>TLLCGEIHYFRVPKHLWRDRLLKLKRAGGNCVSTYIPWNWHDPREKVVNFTDGTSQWHVASYYSRDLASFLELAGELGLRVIARPGPYICSEWDSGGHPNWIYTKAMRLRSLDPGYFKHVVEWYNSVLNILKPYVEREIVIGIQVENEYFWGNEKYIEKLAEIVEEKLPGVLVFTNEDPYLTRIPNTIDLYPSPWDMRQFDDRLRSYLSSQPGLFKMIMELEGGWFKSSRYGYYPTNRLSIPPEWTEILLKTAVGMGLNNINIYMFHGGSNPGYYTAKYLASSYDFEACIREWGELSERYYRVKRVFTFLNGFQELVTSLKPGETVKTASTCSELLQRVGDHGKIAVLRNTGDNLCYQRLINRGEIIPMWTPIRVPPRYAKIVLLDLVVEGTPFKLVYTSGEALLMKRLGDTVVMIIYGDHGEYTETAVEVEGGVLDVDIQGDVLIRREGERAYLVVNHTHGEHLAIVKSTRGQNLLLIFTCRCRAEKTWIVDEDLVLISNIYYIGDSRIDEGKVVINAELDEDSCGRLLVVTSREIEAISLEDLDLDLTRLSKYVYATHIPLSMCRSGKNTYHPLEYRLLEDPVFHTLTSINPSSPLLKNGFYENGIYVYRLRLHLDKKQLGDLLDKHLALIG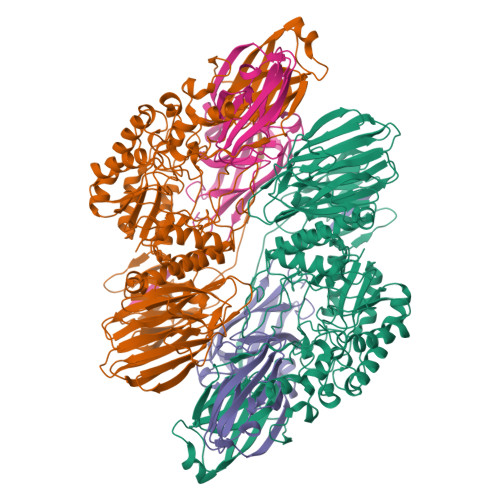FSDYAVVSINNEYAGSGYHYIEMSADSLREGVNEVTVILESTGHPNDGLLYVPNGIYGGVYLGRVGEIRLYKWRKTGFEIPYGPGFDLAEFIANPEPVIKALQE[2x];>ETYSVDSPGLYITEFKVDDLSRHYVLDPGLEFYYNHYYRILLFVNKVYVGPLIGPIDITRYLKPGVNEVALLVEWGVVNPVIGVYQYKVDGEWFIQEGLHGLIEEWFRRSPRGETAEPPILLGDKAGRVIWVNTVIPYEKEPTSSSPVKLEVDFWGCRILVFVNGEFIGRISDDSPERELYVPETAVRRGLNNITLLAIVTSRSSGIRGLRLKETYVHERKEIVFKL[2x]> MGSDKIHHHHHH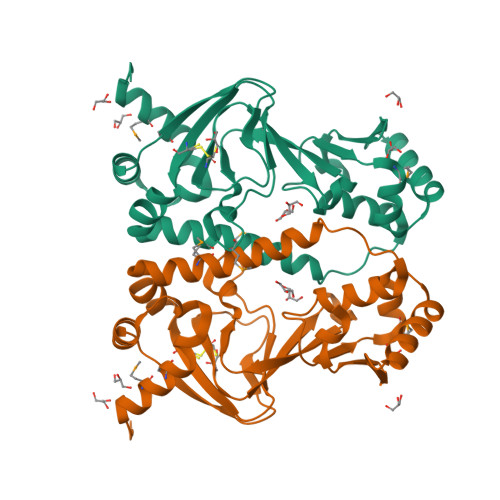METMFDTLLQLPLFQGLCHEDFTSILDKVKLHFIKHKAGETIIKSGNPCTQLCFLLKGEISIVTNAKENIYTVIEQIEAPYLIEPQSLFGMNTNYASSYVAHTEVHTVCISKAFVLSDLFRYDIFRLNYMNIVSNRAQNLYSRLWDEPTLDLKSKIIRFFLSHCEKPQGEKTFKVKMDDLARCLDDTRLNISKTLNELQDNGLIELHRKEILIPDAQKLL> GGC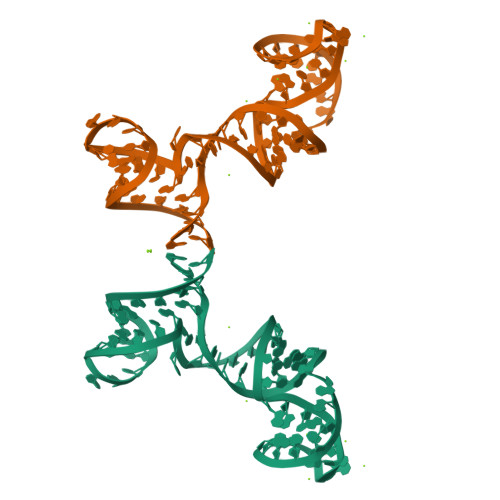GUGUAUGUGGGGAAACCCUGAUUGAGUUCAGCCCACAUACUUUGUUGAUGGUUGUCAAUCGCC> GGLEKDFLPLYFGWFLTKKSSETLRKAGQVFLEELGNHKAFKKELRHFISGDEPKEKLELVSYFGKRPPG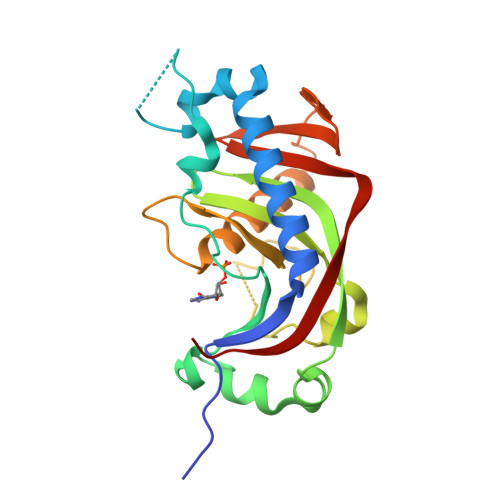VLHCTTKFCDYGKAAGAEEYAQQEVVKRSYGKAFKLSISALFVTPKTAGAQVVLTDQELQLWPSDLDKGSASEGLPPGSRAHVTLGCAADVQPVQTGLDLLDILQQVKGGSQGEAVGELPRGKLYSLGKGRWMLSLTKKMEVKAIFTGYYG> MIHELLLALSGYPGSIFTWNKRGGLQVSQDFPFLHPSETSVLNRLCRLGTDYIRFTEFIEQYTGHVQQQDHHPSQQGQGGLHGIYLRAFCTGLDSVLQPYRQALLDLEQEFLADPHLSISHINYSLDQFQLLFPSVMVVVEQIKSQKIHGCQILETVYKHSCGGLPPVRSALEKILAVCHGVMYKQLSAWMLHGLLLDQHEEFFIKQGPSSGNVSAQPEEDEEDLGIGGLTGKQLRELQDLRLIEEENMLAPSLKQFSLRVEILPSYIPVRVAEKILFVGESVQMFENQNVNLTRKGSILKDQEDTFAAELHRLKQQPLFSLVDFEQVVDRIRSTVAEHLWKLMVEESDLLGQLKIIKDFYLLGRGELFQAFIDTAQHMLKTPPTAVTEHDVNVAFQQSAHKVLLDDDNLLPLLHLTIEYHGKEHKADATQAREGPSRETSPREAPASGWAALGLSYKVQWPLHILFTPAVLEKYNVVFKYLLSVRRVQAELQHCWALQMQRKH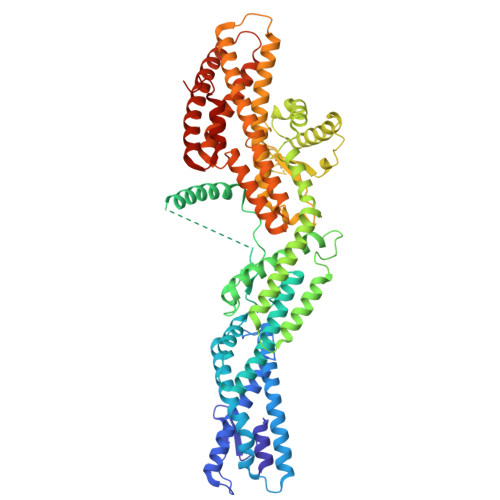LKSNQTDAVKWRLRNHMAFLVDNLQYYLQVDVLESQFSQLLHQINSTRDFESIRLAHDHFLSNLLAQSFILLKPVFHCLNEILDLCHSFCSLVSQNLGPLDERGAAQLSILVKGFSRQSSLLFKILSSVRNHQINSDLAQLLLRLDYNKYYTQAGGTLGSFGM> SSQIRQNYSTEVEAAVNRLVNLYLRASYTYLSLGFYFDRDDVALCGVCAFFHELAEEKREGAERLLKMQNQRGGRALFQDLQKPS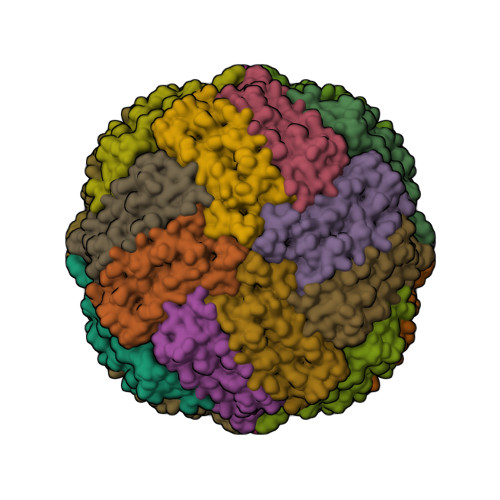QDEWGTTLDAMKAAIVLEKSLNQALLDLHALGSAQADPHLCDFLESHFLDEEVKLIKKMGDHLTNIQRLVGSQAGLGEYLFERLTLKHD> MAEYKDNLLGEANSFLEVLEQVSHLAPLDKPVLIIGERGTGKELIASRLHYLSSRWQGPFISLNCAALNENLLDSELFGHEAGAFTGAQKRHPGRFERADGGTLFLDQLATAPMMVQEKLLRVIEYGELERVGGSQPLQVNVRLVCATNADLPAMVNEGTFRADLLDRLAFDVVQLPPLRERESDIMLMAEYFAIQMCREIKLPLFPGFTERARETLLNYRWPGNIRELKNVVERSVYRHGTSDYPLDDIIIDPFKRRPP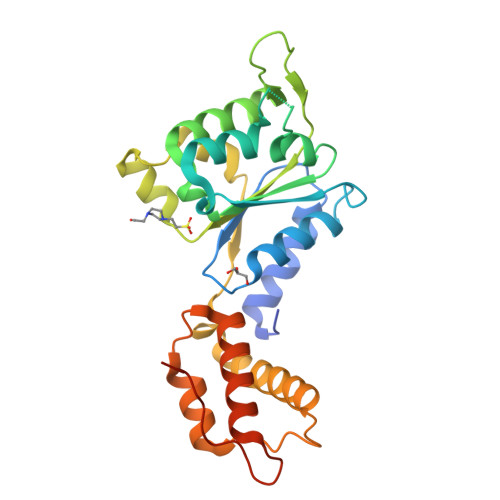EDAIA>[4x]GSRRRAQHNEVERRRRDKINNWIVQLSKIIPDCNADNSKTGASKGGILSKACDYIRELRQTNQRMQETFKEAERLQMDNELLRQQIEELKNENALLRAQLQQHNLEMVGEGTRQ

Upstream stimulating factors (USFs), including USF1 and USF2, are key components of the transcription machinery that recruit coactivators and histone-modifying enzymes. Using the classic basic helix-loop-helix leucine zipper (bHLH-LZ) domain, USFs bind the E-box DNA and form tetramers that promote DNA looping for transcription initiation. USFs belong to the basic helix-loop-helix leucine zipper (bHLH-LZ) transcription factor family, which also includes the MiT/TFE members microphthalmia-associated transcription factor (MITF), transcription factor EB (TFEB), transcription factor EC, and transcription factor E3 (TFE3) and the MYC-subfamily members myc proto-oncogene (MYC), MYC-associated factor X (MAX), MAX dimerization protein, and MAX interacting protein 1 (MXI1). USFs also form a bivalent homotetramer in solution.

To investigate the structure of USF2, we prepared a recombinant protein fragment of human USF2 from the basic region to the C terminus (isoform 1, residues 235–346), including the complete bHLH-LZ domain according to the UniProt database annotation. We cocrystallized this protein with E-box DNA and solved the crystal structure to a resolution of 3.5 Å. One asymmetric unit (ASU) contains four protein chains (A, B, E, and F) and four single strands of DNA (chains C, D, G, and H). Chains A and B as well as E and F form compact dimers to bind duplex E-box DNAs formed in pairs of C and D chains and G and H chains, respectively. In each dimeric USF2-DNA complex, the basic region (from Arg236 to Lys250) forms a helix to bind the major groove of E-box DNA. Interestingly, the rest of the C terminus of one chain of the dimer from Arg329 to Glu342 also forms an α-helix extending LZ (hereafter denoted as the Ext region). LZ-Ext adopts a prominent bent structure with helixes twisted by approximately 125° in both chain A and chain B. Because of the additional leucine spaced seven residues (from Leu321 to Leu328) and the Ext region, the LZ-Ext helix of USF2 is significantly longer than that of other bHLH-LZ transcription factors. In fact, the two dimers further form a compact tetramer in rotational symmetry with a two-fold axis. Finally, we observed that Lys271 in the loop region binds the backbone of G(−7) through a salt bridge.>MISLADLQRRIETGELSPNAAIAQSHAAIEAREKEVHAFVRHDKSARAQASGPLRGIAVGIKDIIDTANMPTEMGSEIYRGWQPRSDAPVVMMLKRAGATIIGKTTTTAFASRDPTATLNPHNTGHSPGGSSSGSAAAVGAGMIPLALGAQTGGSVIRPAAYCGTAAIKPSFRMLPTVGVKCYSWALDTVGLFGARAEDLARGLLAMTGRSEFSGIVPAKAPRIGVVRQEFAGAVEPAAEQGLQAAIKAAERAGASVQAIDLPEAVH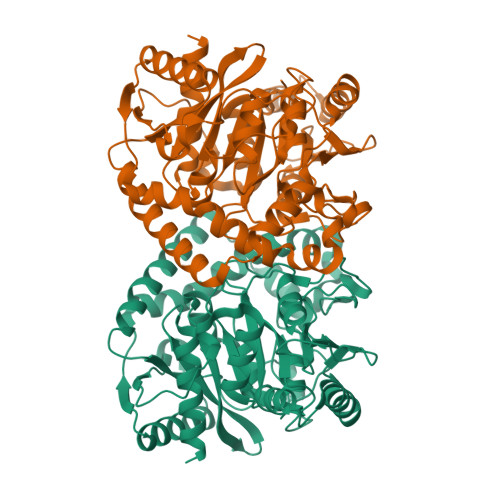EAWRIHPIIQDFEAHRALAWEFSEHHDEIAPMLRASLDATVGLTPKEYDEARRIGRRGRRELGEVFEGVDVLLTYSAPGTAPAKALASTGDPRYNRLWTLMGNPCVNVPVLKVGGLPIGVQVIARFGNDAHALATAWFLEDALAKSG[2x]> ST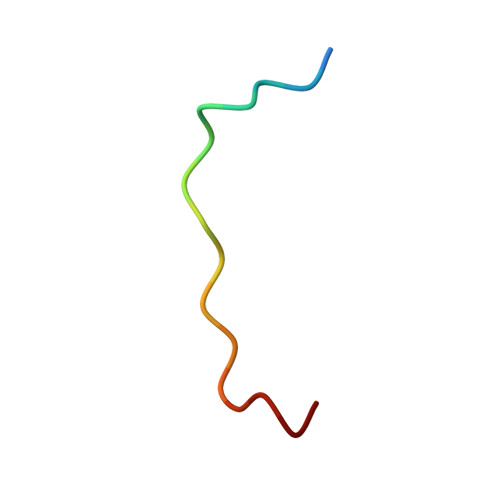LNPNAKEFNPRSFSQ>[4x]SDFANLSSTNKELSPQYNWVACGILEGGLKAAGVLEEGQYNRELAEAIA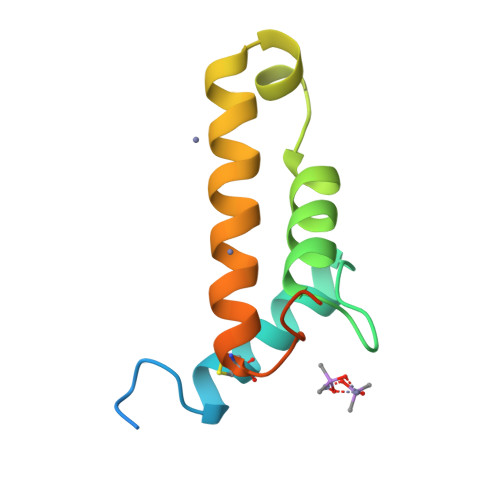AKGEGFWTTQFPQIGDWNEDQAAALADRAQTCGLVKADTYLSELSSNFSS(2R,3S)-2-(3,4-dihydroxyphenyl)-3,4-dihydro-2H-chromene-3,5,7-triol 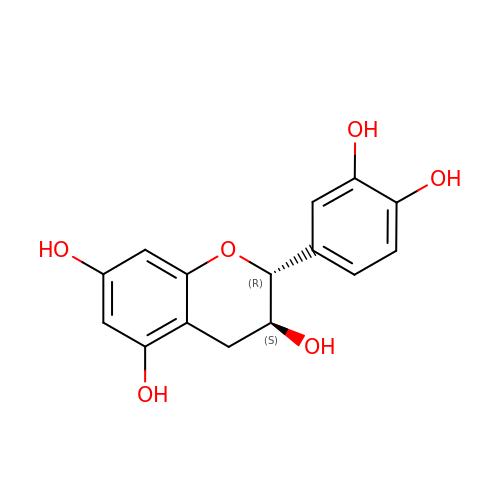| C15 H14 O6 | PFTAWBLQPZVEMU-DZGCQCFKSA-N PLK4, and this interaction targets STIL to centrioles. allows homo-multimerisation, the interaction with the PB3 domain of PLK4, or both. structures and interactions of CCDs and PLK4-PB3s in humans and flies. STIL/Ana2, which can then interact with and recruit Sas-6.

HsPB3 and HsCCD form a complex. heterodimer, i.e. a 2:2 complex (coloured chains). CCD residues interfacing with PB3 are coloured green. highlighting the highly hydrophobic nature of the interaction. previously identified interaction between HsCCD and HsPB3. self-association and binding to PB3 are mutually exclusive events. the PB3 strand-swapped multimer must have undergone a dramatic remodelling.

>GPMGSAQLLKSVFVKNVGWATQLTSGAVWVQFNDGSQLVVQAGVSSISYTSPNGQTTRYGENEKLPDYIKQKLQCLSSILLMFSNPTPNFH[3x];>[3x]GGSLTEQDRQLRLLQAQIQRLLEAQSLM> MLPRVTKLNSRLLSLALLGIQIARGAITYQHP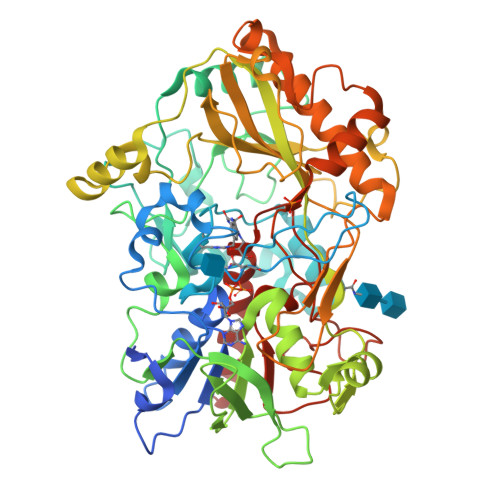DDLPSGVDYDFIVAGGGTAGLVVASRLSENSNWKVLVIEAGPSNKDAFVTRVPGLASTLGAGSPIDWNYTTIPQDGLDGRSLDYPRAKILGGCSTHNGMVYTRGSKDDWNSWAGIIGDQGLGWDSILPAIKKAEKFTQDFTDQSVKGHIDPSVHGFDGKLSVSAAYSNISFNDLLFETTKELNAEFPFKLDMNDGKPIGLGWTQYTIDNHAERSSSATSYLESTGDNVHVLVNTLVTRVLSASGNGTDFRKVEFAVDANSPKKQLEAKKEVIVAGGVIASPQILMNSGIGERKVLQAVGIDTLIDNPSVGKNLSDQGATSVMFDTTLPSTDFDVDAALTEWTNSHTGPLARGARLNHLTFVRLPDDKLNGQDPSSGKNSPHIEFQFAQITPQVPTLGVPKQAPLPAANSYRLLLQLAVVNLYSISRGSISLSDNNPFTYPLIDLNMFKEDIDIAILREGIRSAGRMFSSKAFKNSVNKFVYPPADATSDEDLDAFLRSSTFSYVHGVGTLSMSPKGASWGVVNPDFKVKGTSGLRVVDASVIPHAPAAHTQLPVYAFAEYASALIAKSYN> MSLI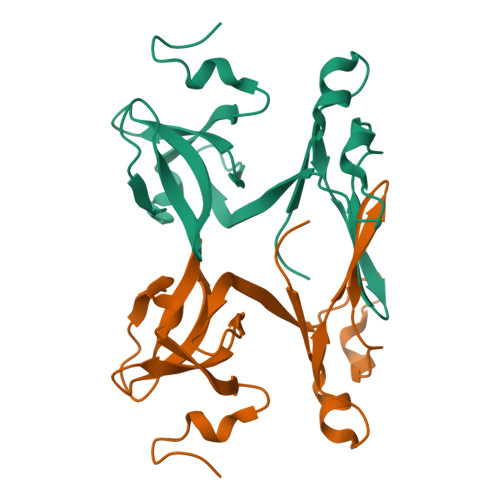PKFREFDRERHRTDYQKGMSYAEQQDFDMGFTIWFDHIEDLDLIEKDGTINRIVMMSTGLKDKNVKEIYESDIVRNLYGELYVVEWLDGSFVLTEFYNGGYDHYIIDSSTEYEVLGNIYENPELLEDDNHASNEGHHHHHH TMEM16 scramblases dissipate the plasma membrane lipid asymmetry to activate multiple eukaryotic cellular pathways. The TMEM16 superfamily is comprised of Cl- channels and dual function scramblases/non-selective ion channels. Our results show afTMEM16 thins the membrane to enable scrambling and that an open hydrophilic pathway is not a structural requirement to allow rapid transbilayer movement of lipids. Scrambling by the TMEM16’s is modulated by two signals, binding of Ca2+ facilitates opening of the groove while the properties of the membrane determine whether the scramblase can thin the membrane enough to enable lipid flipping.

Scrambling by D511A/E514A afTMEM16 is modulated by membrane thickness like the WT protein in 0 Ca2+,  and in C14 membranes its activity is ~30% of that of the WT protein in C18 lipids and saturating Ca2+. To test whether the D511A/E514A afTMEM16 adopts an open-pathway conformation in conditions of high activity, we determined its structure in C14 nanodiscs with 0.5 mM Ca2+ to 3.1 Å resolution. As expected, despite the presence of 0.5 mM Ca2+, the protein adopts the same conformation as in the WT apo structure and there is no density in the Ca2+ binding site. In all reconstructions the permeation pathway is closed, with Cα r.m.s.d. ~1.1 Å to C18/0 Ca2+ and ~0.4 Å to C14/0 Ca2+, indicating that increased scrambling is again not accompanied by higher open probability of the groove. Together, our results suggest that scrambling of afTMEM16 in 0 Ca2+ occurs outside of a closed groove. In the three datasets for apo afTMEM16 (C18/0 Ca2+, C14/0 Ca2+ and DA/EA in 0.5 mM Ca2+) we could resolve 4–9 lipids per monomer, all localized near the dimer interface in positions closely resembling those seen in C18/Ca2+ structure, supporting the notion that these lipids interact strongly with the protein. No lipids could be resolved near the closed pathway in these structures.

>MAFNPAPKAVQENHHVDYVIRFNYGDIDTPEAIKKFEVLLLELSEVGLQTEVRQGDENSLFVFVRAASKKKLKRAVYQSRVRDWLYGVRNTEPEPASSAKPQSEAERLLVIYHLITVPKAEGGAGITPRHGEWKNVDAIFPLHDEETNRQCMREWSKKTFLSTEDLDRIRNTFGEHVGFYFAFLQSYFRFLMFPAAFGFSCWLLLGSFSIIYTVVNCLWCIVFIEYWKRQEEDLSCRWQTKGVSAVHEKRAEFKPEKEIRDESTGEVRGVFPATKRMYRQLLQVPFALLAAVALGAIIATCFAIEIFISEVYNGPLKGYLVFIPTILVSALIPTMSAVLLTVATKLNDYENYETQDAYKVALTQKIFVVNFITSYLPIILTAFVYVPFASRIVPYLDVFHLTVRPFVSKEHAIKARTEFSINPDRLRKQVIYFTVTAQIVGFALETIVPFVKQRVFREYKEYTKKQHAKAEPGNGAGEKKTVSLGDDEDEARFLTRVRNEAELEDYDVTDALRAMCIQFGYLALFSPVWPLVPVSFLINNWVELRSDFFKICVECKRPWPQRADTIGPWLDSLGFLSWVGSITSSALVYMFSNGHEGPNGEPTTIRCWALLLTIFFSEHLYLIVRYAVRSALAKLEPPNTRRERIERFMMRKRYLDTVLSAESDDDADEVKGVVSSIPPSEITRESLEQDARDWSKQGTDPTERFWMRQRGWKESAEVGLSLITKAKGDETKKQQ[2x]> GPAEPALREQQLQQELLALKQKQQIQRQILIAEFQRQHEQLSRQHEAQLHEHIKQQQEMLAMKHQQELLEHQRKLERHRQEQELEK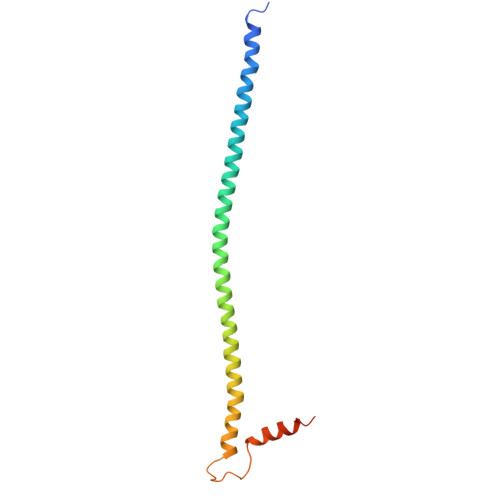QHREQKLQQLKNKEKGKESAVASTEVKMKLQEFVLNKKKALAHRNLN>MRGSHHHHHHGMASHMSSKLVLVLNCGSSSLKFAIIDAVNGDEYLSGLAECFHLPEARI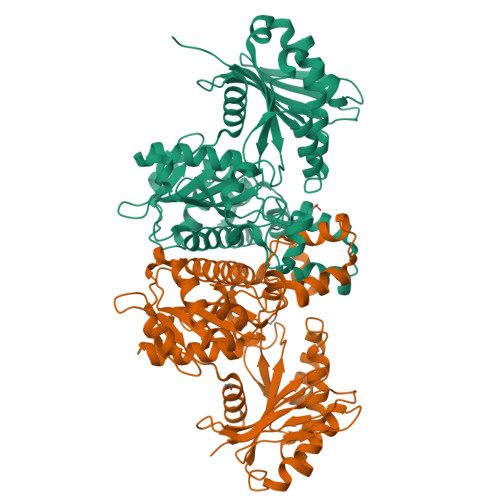KWKMDGSKQEAALGAGAAHSEALNFIVNTILAQKPELSAQLTAIGHRIVHGGEKYTSSVVIDESVIQGIKDSASFAPLHNPAHLIGIAEALKSFPQLKDKNVAVFDTAFHQTMPEESYLYALPYSLYKEHGVRRYGAHGTSHFYVTQEAAKMLNKPVEELNIITCHLGNGGSVSAIRNGKCVDTSMGLTPLEGLVMGTRSGDIDPAIIFHLHDTLGMSVDQINKMLTKESGLLGLTEVTSDCRYVEDNYATKEDAKRAMDVYCHRLAKYIGSYTALMDGRLDAVVFTGGIGENAAMVRELSLGKLGVLGFEVDHERNLAARFGKSGFINKEGTRPAVVIPTNEELVIAQDASRLTA[4x]>MPFITVGQENSTSIDLYYEDHGTGTPVVLIHGFPLSGHSWERQSAALLDAGYRVITYDRRGFGQSSQPTTGYDYDTFAADLNTVLETLDLQDAVLVGFSMGTGEVARYVSSYGTARIAAVAFLASLEPFLLKTDDNPDGAAPQEFFDGIVAAVKADRYAFYTGFFNDFYNLDENLGTRISEEAVRNSWNTAASGGFFAAAAAPTTWYTDFRADIPRIDVPALILHGTGDRTLPIENTARVFHKALPSAEYVEVEGAPHGLLWTHAEEVNTALLAFLAKAQEAQKQKLLTEVETYVLSIIPSGPLKAEIAQRLEDVFAGKNTDLEVLMEWLKTRPILSPLTKGILGFVFTLTVPSERGLQRRRFVQNALNGNGDPNNMDKAVKLYRKLKREITFHGAKEISLSYSAGALASCMGLIY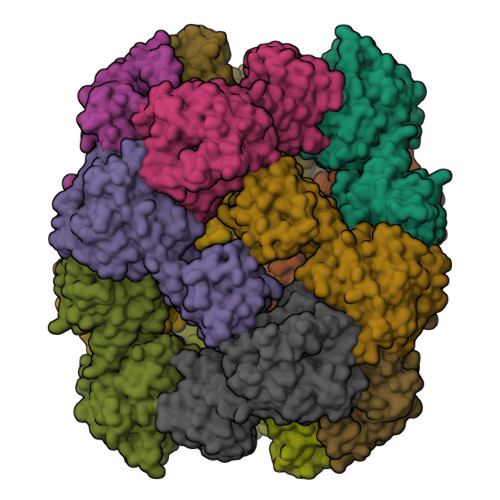NRMGAVTTEVAFGLVCATCEQIADSQHRSHRQLEHHHHHH[6x]>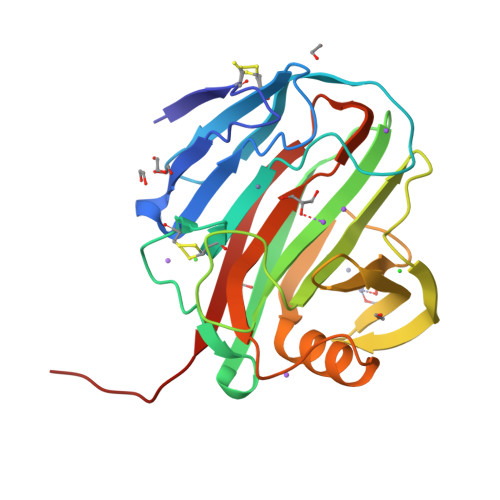 GTTVTDCTPGPNQNGVTSVQGDEYRVQTNEWNSSAQQCLTINTATGAWTVSTANFSGGTGGAPATYPSIYKGCHWGNCTTKNVGMPIQISQIGSAVTSWSTTQVSSGAYDVAYDIWTNSTPTTTGQPNGTEIMIWLNSRGGVQPFGSQTATGVTVAGHTWNVWQGQQTSWKIISYVLTPGATSISNLDLKAIFADAAARGSLNTSDYLLDVEAGFEIWQGGQGLGSNSFSVSVTSGSAHHHHHH>HHHHHHSSGLVPRGSHMRVVVLNWDLLEQVLELGIQPVGAPELSSYVQWVVQPEVPSSVQDIGTRTEPNLEKIAALKPDVILAAGPQQDLLATLGRIAPVVYLPNFSEQDNAAQVAISHFKTLATLFGKEAVAQQKLEAMYARFSELKASLQHAFGDTLPAVVTLRFANPTSVFLYTENSTPQYVLEQLGLSSALPQPPKEWGIV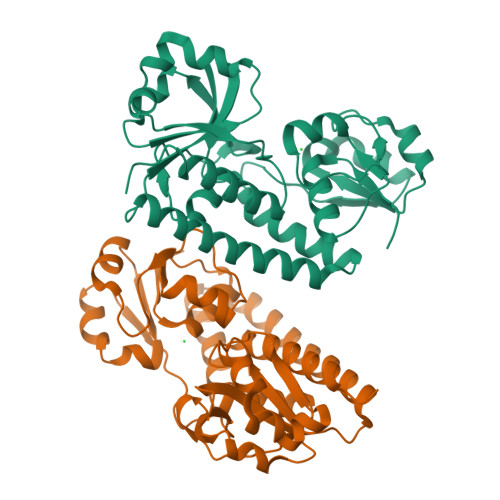QKRLSELQHVEQGYVLYFLPFAEEKKVQKSVLWRAMPFVQAGRVNSVRPVWSYGGAMSLRYSAEAITESLLAVAPQS[2x]> RRRETQ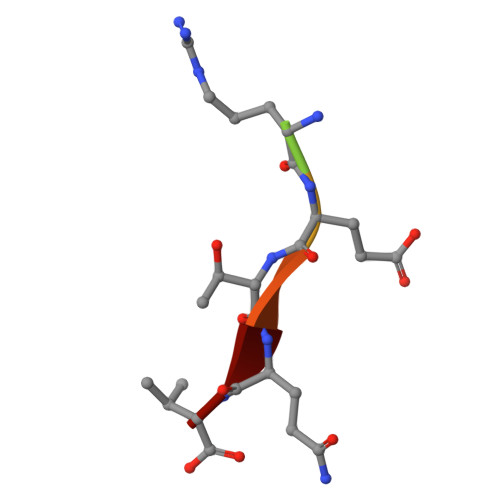V>[2x]MGTSLTDEELVTMSVRELNQHLRGLSKEEIVQLKQRRRTLKNRGYAASCRVKRVTQKEELEKQKAELQQEVEKLASENASMKLELDALRSKYEALQTFARTVAR;>GPHMAHLTRDELRAKALHIPFPVEKIINLPVVDFNEMMSKEQFNEAQLALIRDIRRRGKNKVAAQNCRKRKLENIVELEQDLDHLKDEKEKLLKEKGENDKSLHLLKKQLSTL[2x]

Nuclear factor erythroid 2-like factor (Nrf2/NFE2L2) is a member of the CNC family and plays a central role in cellular defense mechanisms against oxidative and electrophilic stresses. Stabilized Nrf2 then translocates to the nucleus and forms heterodimers with sMaf proteins, thereby functioning as a transcriptional activator and upregulating the target genes involved in anti-stress responses. In this study, we report the crystal structures of Nrf2/NFE2L2, a CNC family protein regulating anti-stress transcriptional responses, in a complex with MafG and CsMBE. The co-crystal structures of Nrf2–MafG-CsMBE complexes show that the CNC motif stabilizes the conformation of Arg residues in the basic region in contact with DNA phosphates.

We solved the crystal structures of the heterodimer between the DNA-binding domains of human Nrf2 (residues 452–560) and MafG (residues 21–123) in complexes with two kinds of DNA fragments containing CsMBE (CsMBE1: 5′-ATGATGAGTCAGCAA-3′ and CsMBE2: 5′-ACAGTGACTCAGCAG-3′, where CsMBE elements are underlined) at 2.3 and 2.6 Å resolutions, respectively. As the CsMBE1-containing complex was solved at a higher resolution, we mainly discuss this complex here, unless otherwise noted. The DNA-binding domain of Nrf2 contains the N-terminal three short α-helices (α1–α3), followed by a large one (α4). The CNC motif (residues 456–498) constitutes the first three helices and a part of α4. Furthermore, α4 contains the basic region (residues 499–518) and the leucine zipper (residues 519–560), which mediate the interactions with DNA and MafG, respectively. Three Nrf2 residues (Asn507, Ala510, and Ala511) recognized the central TRE half site (positions 5–7, 5′-TGA-3′) in a manner similar to that of AP-1 proteins. The N-terminal side of the basic region of Nrf2 has three basic residues that contact DNA phosphates (Arg499, Arg502 and Arg504). Notably, Arg499 of Nrf2 contacts the DNA phosphates up to four nucleotides upstream of the core TRE segment, while no other bZIP protein binds the DNA phosphate at the same position. In the crystal structure, the N7 atom of dA4, which is unique to purine bases, is recognized by Nrf2 Asn507 via water-mediated hydrogen bonds. The bridging water molecule is clearly visible in the electron density map of the CsMBE1 complex structure.> HHHHHHSSGRENLYFQGHMSKLLMIGTGPVAIQLANICYLKSDYEIDMVGRASTSEKSKRLYQAYKKEKQFE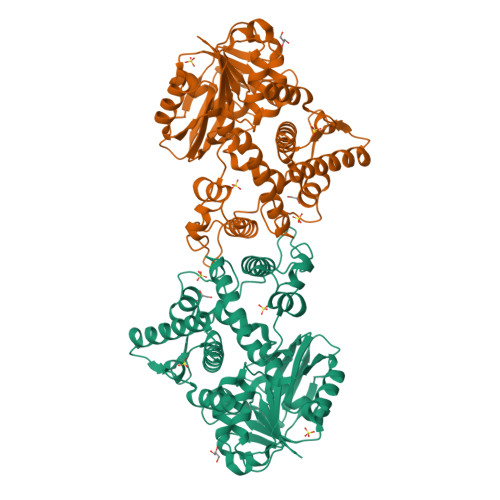VKIQNEAHQHEGKFEINRLYKDVKNVKGEYETVVMACTADAYYDTLQQLSLETLQSVKHVILISPTFGSQMIVEQFMSKFSQDIEVISFSTYLGDTRIVDKEAPNHVLTTGVKKKLYMGSTHSNSTMCQRISALAEQLKIQLEVVESPLHAETRNSSLYVHPPLFMNDFSLKAIFEGTDVPVYVYKLFPEGPITMTLIREMRLMWKEMMAILQAFRVPSVNLLQFMVKENYPVRPETLDEGDIEHFEILPDILQEYLLYVRYTAILIDPFSQPDENGHYFDFSAVPFKQVYKNEQDVVQIPRMPSEDYYRTAMIQHIGKMLGIKTPMIDQFLTRYEASCQAYKDMHQDQQLSSQFNTNLFEGDKALVTKFLEINRTLS> GSDELYRQSLEIISRYLREQATGAKDTKPMGRSGATSRKALETLRRVGDGVQRNHETAFQGMLRKLDIKNEDDVKSLSRVMIHVFSDGVTNWGRIVTLISFGAFVAKHLKTINQESCIEPLAESITDVLVRTKRDWLVKQRGWDGFVEFFHVE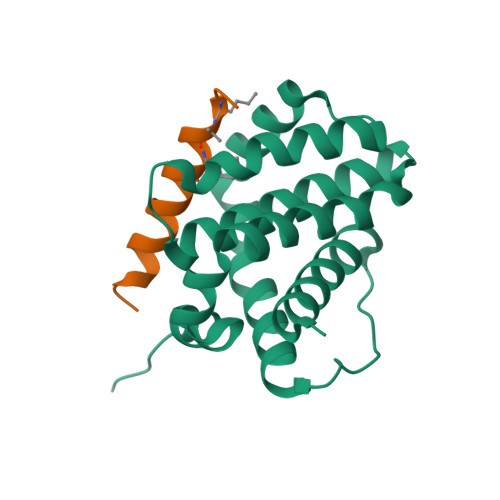DLE;> XIWLAQGGRRLGDEINAYYARRX>[4x]MKTIEVDDELYSYIASHTKHIGESRSDILRRMLKFSAASQKPVKTIKDKVRAMRELLLSDEYAEQKRAVNRFMLLL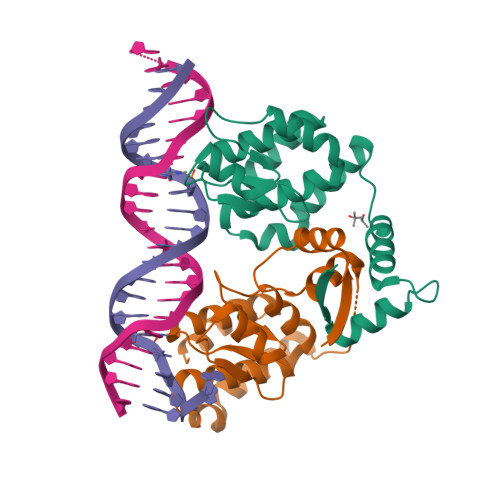STLYSLDAQAFAEATESLHGRTRVYFAADEQTLLKNGNQTKPKHVPGTPYWVITNTNTGRKCSMIEHIMQSMQFPAELIEKVCGTI>[2x]MKKLLFAIDDTEACERAAQYILDMFGKDADCTLTLIHVKPEFMLYGEAVLAAYDEIEMKEEEKAKLLTQKFSTFFTEKG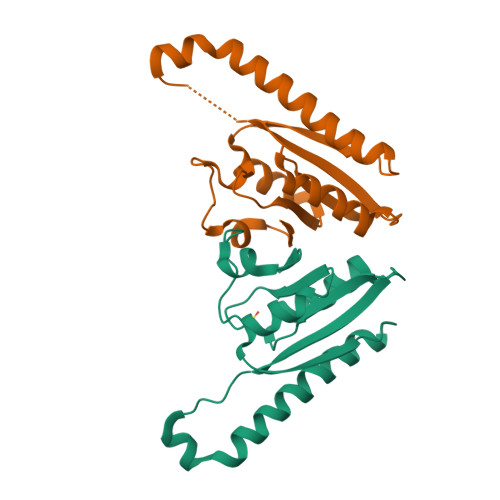INPFVVIKEGEPVEMVLEEAKDYNLLIIGSSENSFLNKIFASHQDDFIQKAPIPVLIVK>MRRRAVLGGAVVYPEGPPPSYESVMQQQAAMIQPPLEAPFVPPRYLAPTEGRNSIRYSELSPLYDTTKLYLVDNKSADIASLNYQNDHSNFLTTVVQNNDFTPTEASTQTINFDERSRWGGQLKTIMHTNMPNVNEYMFSNKFKARVMVSRKAPEGEFVTVNDGPVNDTYDHKEDILKYEWFEFILPEGNFSATMTIDLMNNAIIDNYLEIGRQNGVLESDIGVKFDTRNFRLGWDPETKLIMPGVYTYEAFHPDIVLLPGCGVDFTESR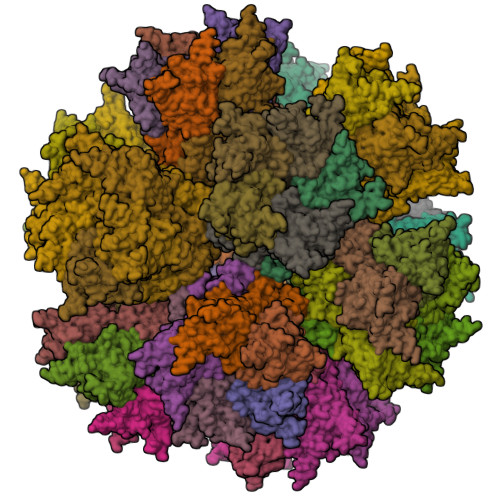LSNLLGIRKRHPFQEGFKIMYEDLEGGNIPALLDVTAYEESKKDTTTARETTTLAVAEETSEDVDDDITRGDTYITELEKQKREAAAAEVSRKKELKIQPLEKDSKSRSYNVLEDKINTAYRSWYLSYNYGNPEKGIRSWTLLTTSDVTCGAEQVYWSLPDMMQDPVTFRSTRQVNNYPVVGAELMPVFSKSFYNEQAVYSQQLRQATSLTHVFNRFPENQILIRPPAPTITTVSENVPALTDHGTLPLRSSIRGVQRVTVTDARRRTCPYVYKALGIVAPRVLSSRTF[60x]>[2x]GSMTEIALIGNPASGKTSLFNLITGHNQRVGNWPGVTVERKSGLVKKNKDLEIQDLPGIYSM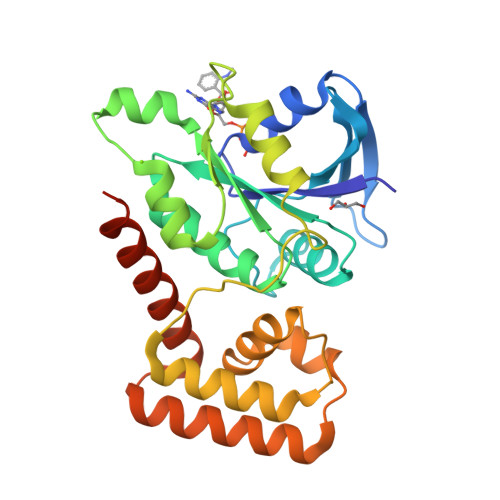SPYSPEEKVARDYLLSQRADSILNVVDATNLERNLYLTTQLIETGIPVTIALNMIDVLDGQGKKINVDKLSYHLGVPVVATSALKQTGVDQVVKKAAHTTTSTVGDLAFPIYDDRLEAAISQILEVLGNSVPQRSARFYAIKLFEQDSLVEAELDLSQFQRKEIEDIIRITEEIFTEDAESIVINERYAFIERVCQMAESHTEDFALTLS>[4x]VPDPTSAIGVLTSGGDAQGMNAAVRAVVRMGIYVGAKVYFIYEGYQGMVDGGSNIAEADWESVSSILQVGGTIIGSARCQAFRTREGRLKAACNLLQRGITNLCVIGGDGSLTGANLFRKEWSGLLEELARNGQIDKEAVQKYAYLNVVGMVGSIDNDFCGTDMTIGTDSALHRIIEVVDAIMTTAQSHQRTFVLEVMGRHCGYLALVSALACGADWVFLPESPPEEGWEEQMCVKLSENRARKKRLNIIIVAEGAIDTQNKPITSEKIKELVVTQLGYDTRVTILGHVQRGGTPSAFDRILASRMGVEAVIALLEATPDTPACVVSLNGNHAVRLPLMECVQMTQDVQKAMDERRFQDAVRLRGRSFAGNLNTYKRLAIKLPDDQIPKTNCNVAVINVGAPAAGMNAAVRSAVRVGIADGHRMLAIYDGFDG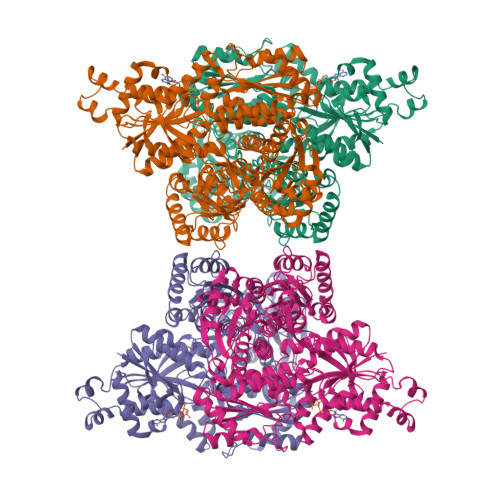FAKGQIKEIGWTDVGGWTGQGGSILGTKRVLPGKYLEEIATQMRTHSINALLIIGGFEAYLGLLELSAAREKHEEFCVPMVMVPATVSNNVPGSDFSIGADTALNTITDTCDRIKQSASGTKRRVFIIETMGGYCGYLANMGGLAAGADAAYIFEEPFDIRDLQSNVEHLTEKMKTTIQRGLVLRNESCSENYTTDFIYQLYSEEGKGVFDCRKNVLGHMQQGGAPSPFDRNFGTKISARAMEWITAKLKEARGRGKKFTTDDSICVLGISKRNVIFQPVAELKKQTDFEHRIPKEQWWLKLRPLMKILA> ATCDDGRTTANAACCILFPILDDIQENLFDGAQCGEEVHESLRLTFHDAIGFSPTLGGGGADGSIIAFSDIETNFPANAGIDEIVEAQKPFVAKHNISAGDFIQFAGAVGVSNCPGGVRIPFFLGRPDAVAASPDHLVPEPFDSVTSILARMGDAGFSPVEVVWLLASHSIAAADKVDPSIPGTPFDSTPGVFDSQFFIETLLKGRLFPGTADNKGEAQSPLQGEIRLQSDELLARDPRTACEWQSMVNNQPKIQNRFAATMSKMALLGQDKTKLIDCSDVIPTPPALVGAAHLPAGFSLKDVEQACAATPFPALTADPGPVTSVPPVPGS

Versatile peroxidase (VP, EC 1.11.1.16) constitutes the third family of ligninolytic peroxidases, which was described 20-years ago. VP combines catalytic properties of the above two families due to the presence of both a Mn-oxidation site and a catalytic tryptophan in its molecular structure. In the present work, VP (isoenzyme VPL2) from Pleurotus eryngii has been subjected to protein engineering using a rational design strategy.

Based on these observations and considering that most ion pairs have a stabilizing role, a VP variant (VPi) containing eight substitutions (D69S/T70D/S86E/D146T/Q202L/H232E/Q239R/S301K) was engineered by introducing the residues involved in these interactions in the four targeted regions. Region A (containing mutations D69S/T70D/S86E) is located at the heme distal side above the heme plane, whereas regions B, C and D (containing mutations D146T/Q239R, Q202L/H232E and S301K, respectively) are found at the proximal side below the heme plane. The three mutations introduced in region A fail to emulate the contacts identified in MnP4 (left). However, compared with the native VP (middle), they contribute to reinforce the interaction between helices B'b and C by increasing the H-bond network in this area, as shown in the crystal structure (right). Similarly, the two substitutions in region B strengthen the loop between helices H and I by interaction of the Arg239 guanidinium group with the Asp237 carboxylate (right), mimicking that observed between Arg245 and Asp243 in MnP4 (left). Regarding the region C, the introduction of a glutamate at position 232 in helix H promotes the formation of a salt bridge between this amino acid and Arg227 (right) emulating that observed between Glu238 and Arg233 in MnP4 (left). By contrast, the side-chain of Lys301 appears exposed to the solvent. Summarizing, three of the four protein regions containing mutations exhibit a modified distribution of hydrogen bonds and salt bridges that can be correlated with the improvement in pH stability previously described for the VPi variant. The results revealed that VPi is significantly more stable than native VP at acidic and neutral pH.>[5x]MTTRKESELEGVTLLGNQGTNYLFEYAPDVLESFPNKHVNRDYF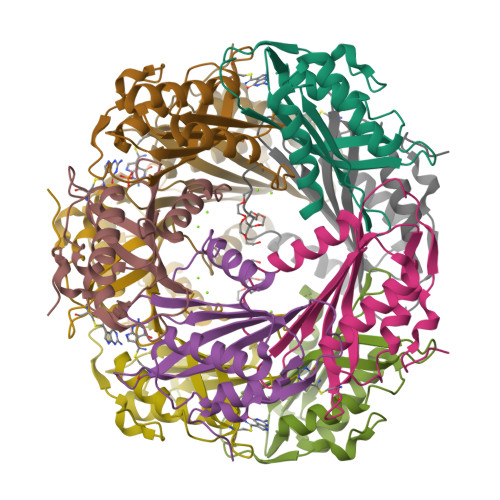VKFNCPEFTSLCPKTGQPDFATIYISYIPDEKMVESKSLKLYLFSFRNHGDFHEDCMNIIMNDLIELMDPRYIEVWGKFTPRGGISIDPYTNYGKPGTKYEKMAEYRMMNHDLYPETIDNR>MCTAITLNGNSNYFGRNLDLDFSYGEEVIITPAEYEFKFRKEKAIKNHKSLIGVGIVANDYPLYFDAINEDGLGMAGLNFPGNAYYSDALENDKDNITPFEFIPWILGQCSDVNEARNLVEKINLINLSFSEQLPLAGLHWLIADREKSIVVEVTKSGVHIYDNPIGILTNNPEFNYQMYNLNKYRNLSISTPQNTFSDSVDLKVDGTGFGGIGLPGDVSPESRFVRATFSKLNSSKGMTVEEDIT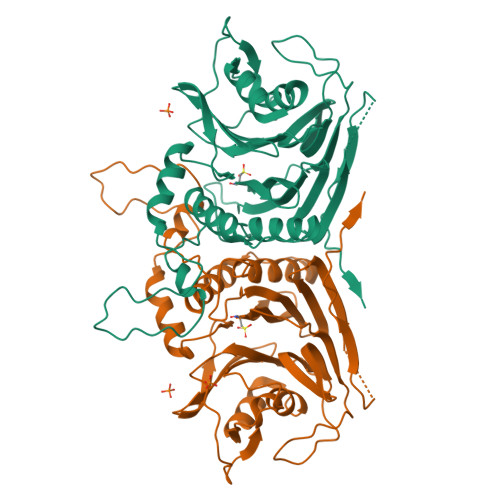QFFHILGTVEQIKGVNKTESGKEEYTVYSNCYDLDNKTLYYTTYENRQIVAVTLNKDKDGNRLVTYPFERKQIINKLNLERHHHHHH[2x]> AAPGKPTIAWGNTKFAIVEVDQAATAYNNLVKVKNAADVSVSWNLWNGDTGTTAKVLLNGKEAWSGPSTGSSGTANFKVNKGGRYQMQVALCNADGCTASDATEIVVADTDGSHLAPLKEPLLEKNKPYKQNSGKVVGSYFVEWGVYGRNFTVDKIPAQNLTHLLYGFIPICGGNGINDSLKEIEGSFQALQRSCQGREDFKVSIHDPFAALQKAQKGVTAWDDPYKGNFGQLMALKQAHPDLKILPSIGGWTLSDPFFFMGDK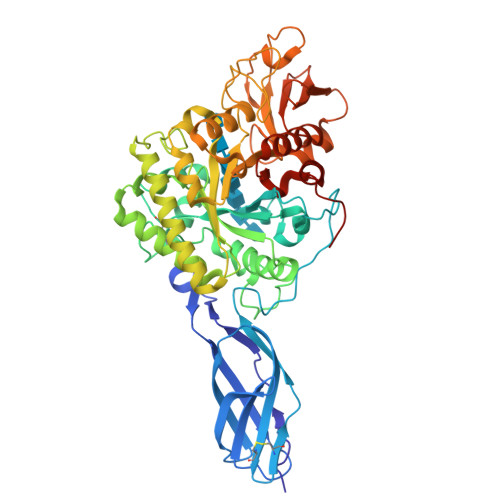VKRDRFVGSVKEFLQTWKFFDGVDIDWQFPGGKGANPNLGSPQDGETYVLLMKELRAMLDQLSVETGRKYELTSAISAGKDKIDKVAYNVAQNSMDHIFLMSYDFYGAFDLKNLGHQTALNAPAWKPDTAYTTVNGVNALLAQGVKPGKIVVGTAMYGRGWTGVNGYQNNIPFTGTATGPVKGTWENGIVDYRQIAGQFMSGEWQYTYDATAEAPYVFKPSTGDLITFDDARSVQAKGKYVLDKQLGGLFSWEIDADNGDILNSMNASLGNSAGVQ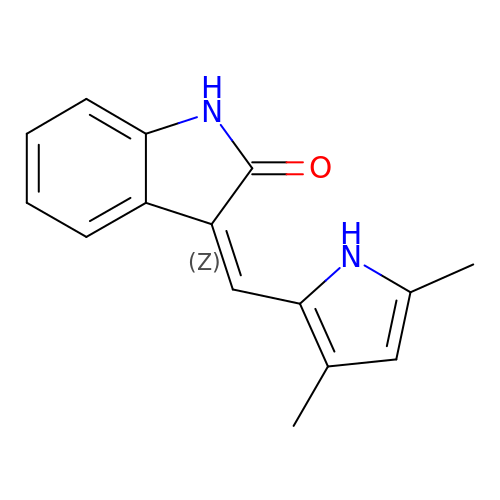(3Z)-3-[(3,5-DIMETHYL-1H-PYRROL-2-YL)METHYLIDENE]-1,3-DIHYDRO-2H-INDOL-2-ONE | C15 H14 N2 O | WUWDLXZGHZSWQZ-WQLSENKSSA-N> MDFLDSLIWERVVDDQYVTNPTFCISDYFEIVRQPGDGNCFYHSIAELFFDVKTPFSFRKVKEHLRLAADAFYDTEPEAIGTGVTKEEYIQAAMKDNEWG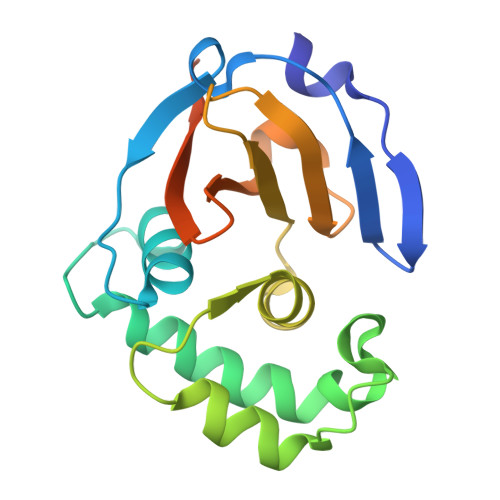GSLEASMLSKQLQITIILWVVNQTEQVTAAIKFGPGRVSTALNLMHVGRTHFDALRVINQLEDNQLQSRSGSHHHHHH>[2x]MQDITMQWYQQLQDASMQCVLTFEGLTNSKDSQAKKIKMDLQKAATIPVSQISTIAGSKLKE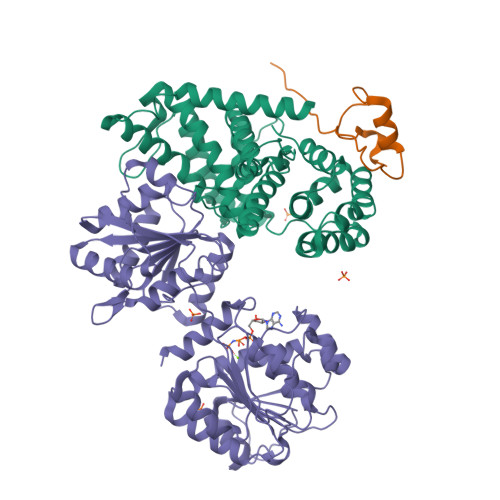IFDKIHSLLSGKPVQSGGRSVSVTLNPQGLDFVQYKLAEKFVKQGEEEVASHHEAAFPIAVVASGIWELHPRVGDLILAHLHKKCPYSVPFYPTFKEGMALEDYQRMLGYQVKDSKVEQQDNFLKRMSGMIRLYAAIIQLRWPYGNRQEIHPHGLNHGWRWLAQILNMEPLSDVTATLLFDFLEVCGNALMKQYQVQFWKMLILIKEDYFPRIEAITSSGQMGSFIRLKQFLEKCLQHKDIPVPKGFLTSSFWRS;>[2x]GPSGSIIATDNVLFTPRDKLTVEELEQFQSKKFTLGKIPLKPPPLELLN;>GPHMEDRAAQSLLNKLIRSNLVDNTNQVEVLQRDPNSPLYSVKSFEELRLKPQLLQGVYAMGFNRPSKIQENALPLMLAEPPQNLIAQSQSGTGKTAAFVLAMLSQVEPANKYPQCLCLSPTYELALQTGKVIEQMGKFYPELKLAYAVRGNKLERGQKISEQIVIGTPGTVLDWCSKLKFIDPKKIKVFVLDEADVMIATQGHQDQSIRIQRMLPRNCQMLLFSATFEDSVWKFAQKVVPDPNVIKLKREEETLDTIKQYYVLCSSRDEKFQALCNLYGAITIAQAMIFCHTRKTASWLAAELSKEGHQVALLSGEMMVEQRAAVIERFREGKEKVLVTTNVCARGIDVEQVSVVINFDLPVDKDGNPDNETYLHRIGRTGRFGKRGLAVNMVDSKHSMNILNRIQEHFNKKIERLDTDDLDEIEKIAN[2x]> ASAPIGSAISRNNWAVTCDSAQSGNECNKAIDGNKDTFWHTFYGANGDPKPPHTYTIDMKTTQNVNGLSMLPRQDGNQNGWIGRHEVYLSSDGTNWGSPVASGSWFADSTTKYSNFETRPARYVRLVAITEANGQPWTSIAEINVFQASSYTAPQPGLGRWGPTIDLPIVPAAAAIEPTSGRVLMWSSYRNDAFGGSPGGITLTSSWDPSTGIVSDRTVTVTKHDMFCPGISMDGNGQIVVTGGNDAKKTSLYDSSSDSWIPGPDMQVARGYQSSATMSDGRVFTIGGSHSGGVFEKNGEVYSPSSKTWTSLPNAKVNPMLTADKQGLYRSDNHAWLFGWKKGSVFQAGPSTAMNWYYTSGSGDVKSAGKRQSNRGVAPDAMCGNAVMYDAVKGKILTFGGSPDYQDSDATTNAHIITLGEPGTSPNTVFASNGLYFARTFHTSVVLPDGSTFITGGQRRGIPFEDSTPVFTPEIYVPEQDTFYKQNPNSIVRVYHSISLLLPDGRVFNGGGGLCGDCTTNHFDAQIFTPNYLYNSNGNLATRPKI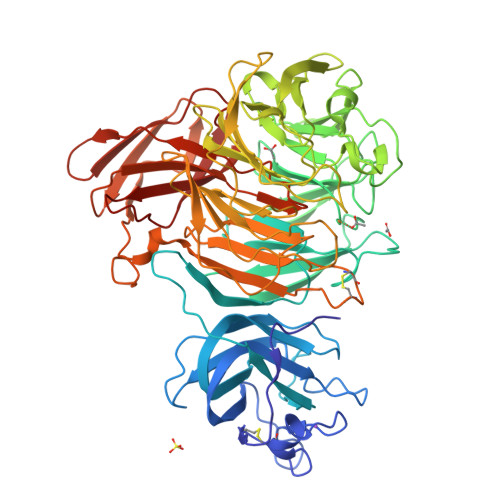TRTSTQSVKVGGRITISTDSSISKASLIRYGTATHTVNTDQRRIPLTLTNNGGNSYSFQVPSDSGVALPGYWMLFVMNSAGVPSVASTIRVTQ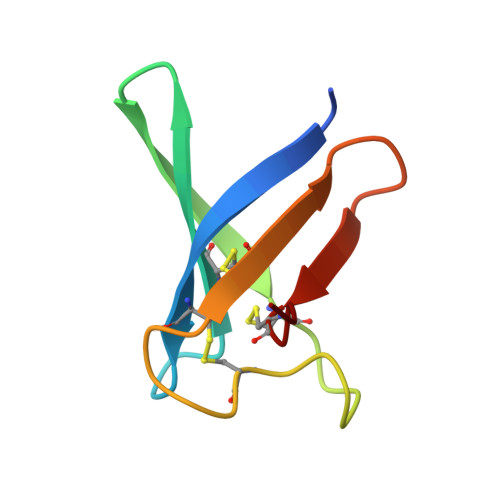> PGLSKFGGECSLKHNTCTYLKGGKNHVVNCGSAANKKCKSDRHHCEYDEHHKRVDCQTPV> MGDDARIAAIGDVDELNSQIGVLLAEPLPDDVRAALSAIQHDL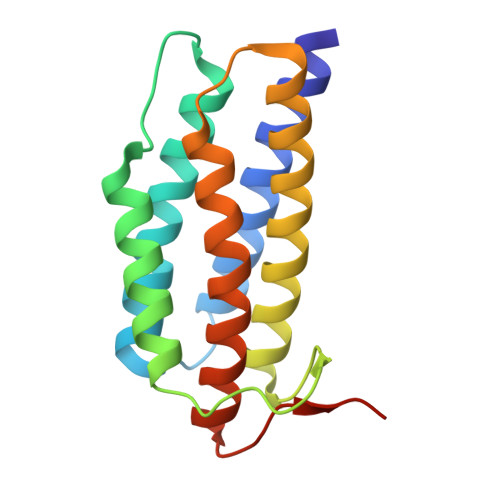FDLGGELCIPGHAAITEDHLLRLALWLVHYNGQLPPLEEFILPGGARGAALAHVCRTVCRRAERSIKALGASEPLNIAPAAYVNLLSDLLFVLARVLNRAAGGADVLWDRTRAH>[4x]MPKRTDIKSILILGAGPIVIGQACEFDYSGAQACKALREEGYRVINVNSNPATIMTDPEMADATYIEPIHWEVVRKIIEKERPDAVLPTMGGQTALNCALELERQGVLEEFGVTMIGATADAIDKAEDRRRFDVAMKKIGLETARSGIAHTMEEALAVAADVGFPCIIRPSFTMGGSGGGIAYNREEFEEICARGLDLSPTKELLIDESLIGWKEYEMEVVRDKNDNCIIVCSIENFDAMGIHTGDSITVAPAQTLTDKEYQIMRNASMAVLREIGVETGGSNVQFAVNPKNGRLIVIEMNPRVSRSSALASKATGFPIAKVAAKLAVGYTLDELMNDITGGRTPASFEPSIDYVVTKIPRFNFEKFAGANDRLTTQMKSVGEVMAIGRTQQESLQKALRGLEVGATGFDPKVSLDDPEALTKIRRELKDAGADRIWYIADAFRAGLSVDGVFNLTNIDRWFLVQIEELVRLEEKVAEVGITGLNADFLRQLKRKGFADARLAKLAGVREAEIRKLRDQYDLHPVYKRVDTCAAEFATDTAYMYSTYEEECEANPSTDREKIMVLGGGPNRIGQGIEFDYCCVHASLALREDGYETIMVNCNPETVSTDYDTSDRLYFEPVTLEDVLEIVRIEKPKGVIVQYGGQTPLKLARALEAAGVPVIGTSPDAIDRAEDRERFQHAVERLKLKQPANATVTAIEMAVEKAKEIGYPLVVRASYVLGGRAMEIVYDEADLRRYFQTAVSVSNDAPVLLDHFLDDAVEVDVDAICDGEMVLIGGIMEHIEQAGVHSGDSACSLPAYTLSQEIQDVMRQQVQKLAFELQVRGLMNVQFAVKNNEVYLIEVNPRAARTVPFVSKATGVPLAKVAARVMAGKSLAEQGVTKEVIPPY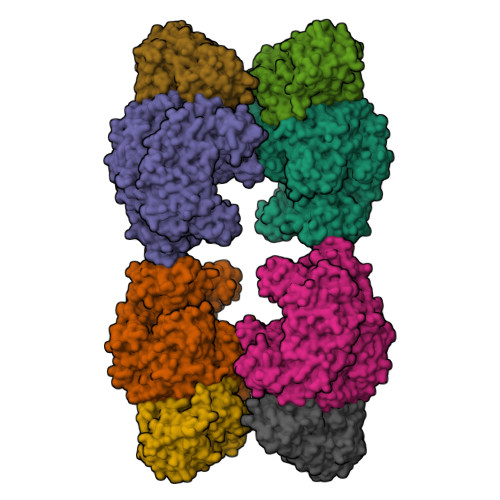YSVKEVVLPFNKFPGVDPLLGPEMRSTGEVMGVGRTFAEAFAKAQLGSNSTMKKHGRALLSVREGDKERVVDLAAKLLKQGFELDATHGTAIVLGEAGINPRLVNKVHEGRPHIQDRIKNGEYTYIINTTSGRRAIEDSRVIRRSALQYKVHYDTTLNGGFATAMALNADATEKVISVQEMHAQIK;>IKSALLVLEDGTQFHGRAIGATGSAVGEVVFNTSMTGYQEILTDPSYSRQIVTLTYPHIGNVGTNDADEESSQVHAQGLVIRDLPLIASNFRNTEDLSSYLKRHNIVAIADIDTRKLTRLLREKGAQNGCIIAGDNPDAALALEKARAFPGLNGMDLAKEVTTAEAYSWTQGSWTLTGGLPQAKKEDELPFHVVAYDFGAKRNILRMLVDRGCRLTIVPAQTSAEDVLKMNPDGIFLSNGPGDPAPCDYAITAIQKFLETDIPVFGICLGHQLLALASGAKTVKMKFGHHGGNHPVKDVEKNVVMITAQNHGFAVDEATLPANLRVTHKSLFDGTLQGIHRTDKPAFSFQGNPEASPGPHDAAPLFDHFIELIEQYRKT[4x]> MKKYVCTVCG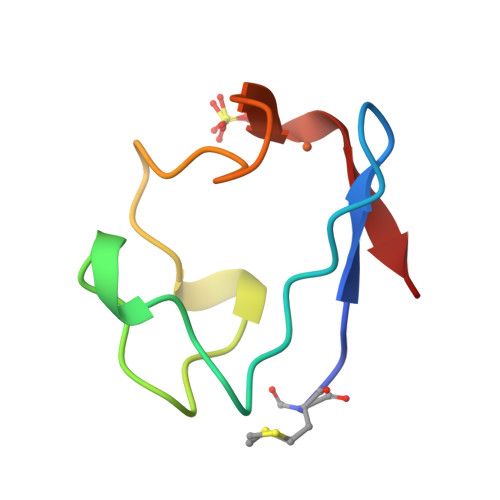YEYDPAEGDPDNGVKPGTSFDDLPADWVCPVCGAPKSEFEAA> MSVDPMTYEAQFFGFTPQTCMLRIYIAFQDYLFEVMQAVEQVILKKLDGIPDCDISPVQIRKCTEKFLCFMKGHFDN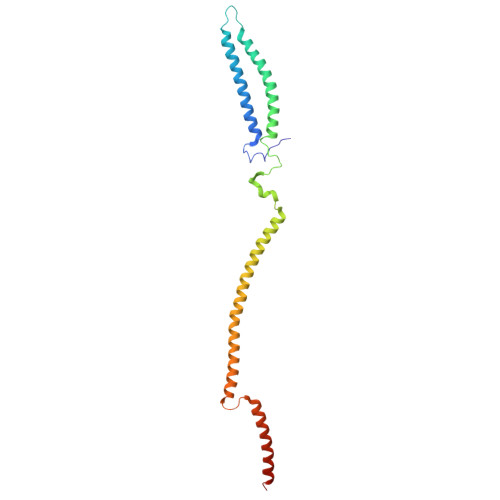LFSKMEQLFLQLILRIPSNILLPEDKCKETPYSEEDFQHLQKEIEQLQEKYKTELCTKQALLAELEEQKIVQAKLKQTLTFFDELHNVGRDHGTSDFRESLVSLVQNSRKLQNIRDNVEKESKRLKIS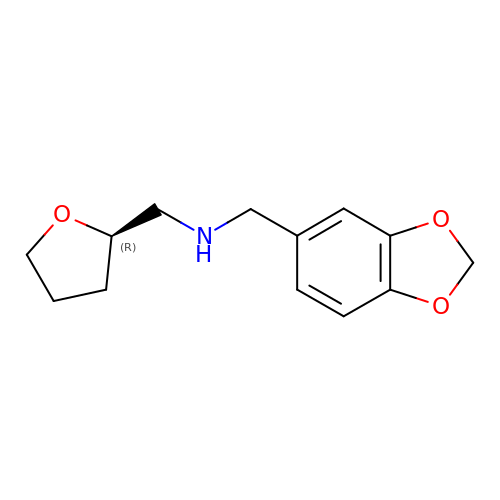1-(1,3-benzodioxol-5-yl)-~{N}-[[(2~{R})-oxolan-2-yl]methyl]methanamine | C13 H17 N O3 | GSKKKMLEVJZIAD-LLVKDONJSA-N> AATSRTERIWPGGVIPYVIGGNFTGSQRAMFKQAMRHWEKHTCVTFIERSDEESYIVFTYRPCGCCSYVGRRGNGPQAISIGKNCDKFGIVVHELGHVIGFWHEHTRPDRDNHVTIIRENIQPGQ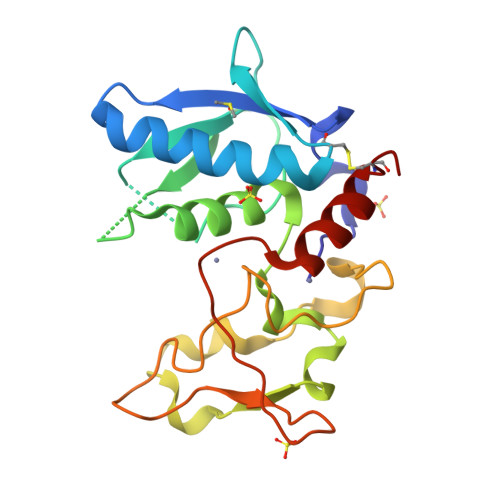EYNFLKMEPGEVNSLGERYDFDSIMHYARNTFSRGMFLDTILPSRDDNGIRPAIGQRTRLSKGDIAQARKLYRCPA> MEGDIHMQENMLKISGYPGMLNTFGIAQLLTPYRVNGITMTGAQS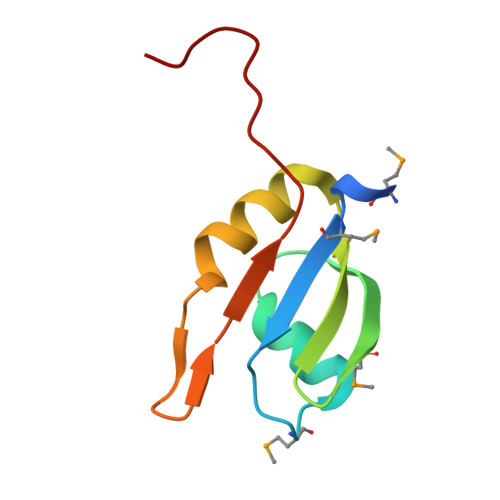AVVALENKFQVYQAVQDFNGKKLDRNHKLQVSSLVVSSPAVPLE> GSTAQARDEQYRNFLRSVSLLKNLPEDKLTKIIDCLEVEYY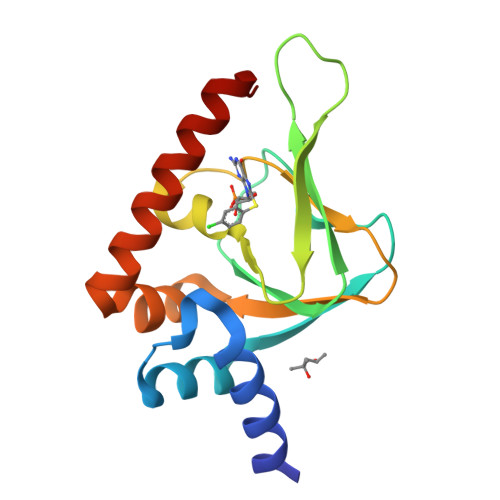DKGDYIIREGEEGSTFFILAKGKVKVTQSTEGHDQPQLIKTLQKGEYFGEKALISDDVRSANIIAEENDVACLVIDRETFNQTVGTFEELQKYLEGYVANLNRDDEKRHAK> GMAAVDSVAQALAYLQVHSPQDGTSMYDHLVKLVSKVLEDQPKNAVDLLETSLLVKKSTFDPKESSPLVPIPVAPDATQTQAAVSIFGDPELPINPATGEPVPADPPNEFEAENMLGAAAVLDCLGVGLGRELGVNIALAAKRIGEDPKLAVRSVRFFGKFLGLYSDYFVFEVAFKKEAAKEAAPAAPAPERVEGEAASSSAPEVPVEEPGKGANKFTYLVCSSLGGP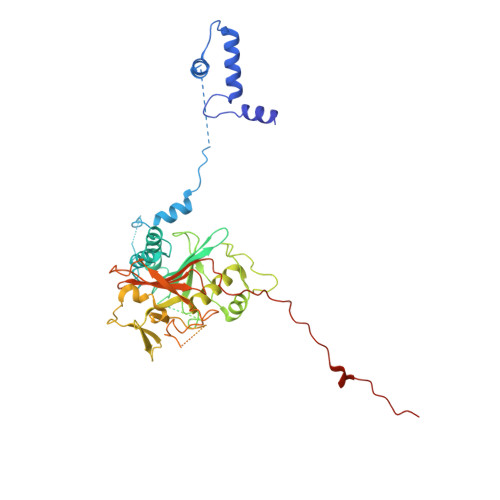LTRLPDVTPAQVKASRRIKKLLTGRLTSHVSTYPAFPGNEANYLRALIARISAATVVAPSDLFSLNDETGELERAEDWEPPAGREMAAPTAWVHVRPHLKSQGRCEVHKRELPEDADEDEFYNEDELEEGPDLLAALEEDAQLPGEQAAWTPIYSSASEAVKTQAGGLRSLVWPGAVCGGRGSEWTCVYVGWGVKNAPFVPLPPPPVAQEFAWGEVETQELELKPAPPPPEEEAEADE>PVPKHIREALQNVHEEVALRYYGCGLVIPEHLENCWILDLGSGSGRDCYVLSQLVGEKGHVTGIDMTKGQVEVAEKYLDYHMEKYGFQASNVTFIHGYIEKLGEAGIKNESHDIVVSNCVINLVPDKQQVLQEAYRVLKHGGELYFSDVYTSLELPEEIRTHKVLWGECLGGALYWKELAVLAQKIGFCPPRLVTANLITIQNKELERVIGDCRFVSATFRLFKHSKTGPTKRCQVIYNGGITGHEKELMFDANFTFKEGEIVEVDEETAAILKNSRFAQDFLIRPIGEKLPTSGGCSALELKDIITDP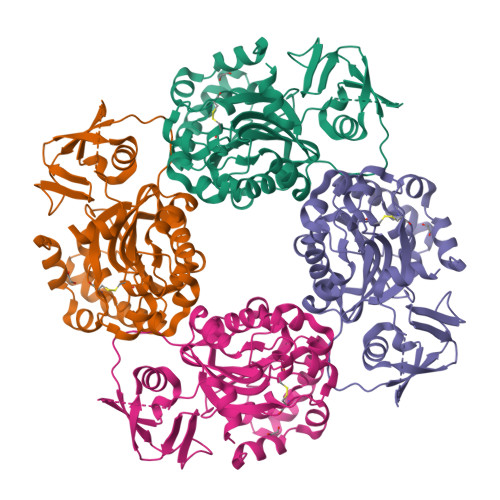FKLAEESDSMKS[4x]> RGHMPPLTSAQQALTGTI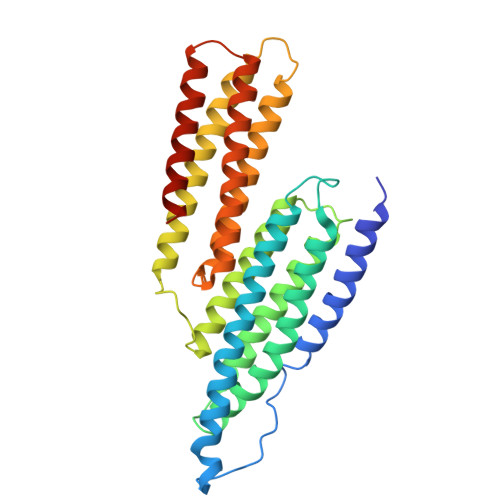NSSMQAVQAAQATLDDFETLPPLGQDAASKAWRKNKMDESKHEIHSQVDAITAGTASVVNLTAGDPAETDYTAVGCAVTTISSNLTEMSRGVKLLAALLEDEGGNGRPLLQAAKGLAGAVSELLRSAQPASAEPRQNLLQAAGNVGQASGELLQQIGESDTDPHFQDVLMQLANAVASAAAALVLKAKSVAQRTEDSGLQTQVIAAATQCALSTSQLVACTKVVAPTISSPVCQEQLVEAGRLVAKAVEGCVSASQAATEDGQLLRGVGAAATAVTQALNELLQHVKAHA>[2x]GSHMDGHIYAVGGFDGHTHLNSVEAYDPERDEWHLVAPMTTRRSGVGVAVLQGRIYVLGGYDGHTFLDSVEAYDPDTDTWSEVTRMTSGRSGVGVAVTDGHIYAVGGFDGHTHLNSVEAYDPERDEWHLVAPMTTRRSGVGVAVLQGRIYVLGGYDGHTFLDSVEAYDPDTDTWSEVTRMTSGRSGVGVAVTDGHIYAVGGFDGHTHLNSVEAYDPERDEWHLVAPMTT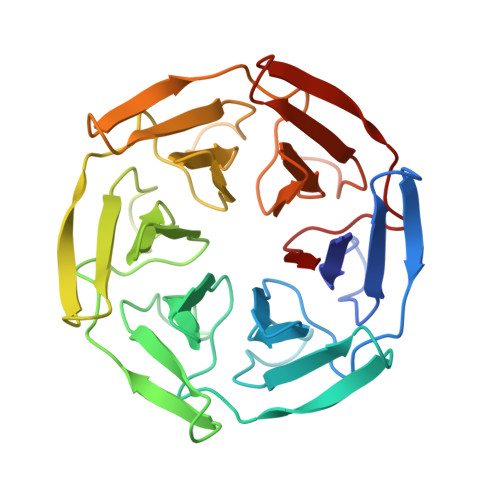RRSGVGVAVLQGRIYVLGGYDGHTFLDSVEAYDPDTDTWSEVTRMTSGRSGVGVAVT> MIYMTFGEILKKERVSWKLSVKELSTLSGVSQTYISKLENGKRNFPSLETIFNLLIGFKTHIEYKMGSESPFYEINNSYLDEILIMFINSSNSTISDRDPNELITQFNEYYDVTIKKKQNENSKIESDIFSNKIKLVKGTTKKEVIEKPYFDLNWLLTQNEYEVFFDRSFLLDNNFLNKKHFTE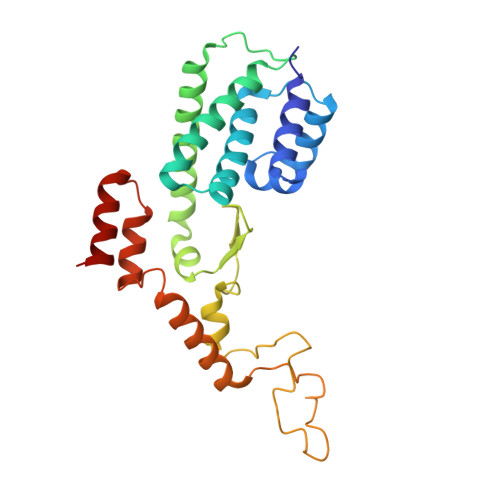KDMYYYNVLNDNDLKTIKDEIVVFLLNKYNYIKNKDDFFNIFTNSEDDKTKRDALYKILYETD> MGYYDDDAHGHVEADAAPRATTGTGTGSASQTVTIPCHHIRLGDILILQGRPCQVIRISTSAATGQHRYLGVDLFTKQLHEESSFVSNPAPSVVVQTMLGPVFKQYRVLDMQDGSIVAMTETGDVKQNLPVIDQSSLWNRLQKAFESGRGSVRVLVVSDHGREMAVDMKVVHGSRLA

Here, we present InCellCryst, an advanced pipeline for producing homogeneous microcrystals directly within living insect cells. We have demonstrated the pipeline on five different proteins (IMPDH, HEX-1, Cathepsin B, Luciferase and EGFP-µNS), representing a selection of soluble proteins of different source organisms that crystallize in insect cells in their native compartment or, in case of peroxisomes, readily in the cytoplasm or nucleus of the cells. Importantly, as shown for IMPDH and HEX-1, InCellCryst can produce crystals from native protein sequences, without purification tags or even remnants of proteolytically removed tags, within a quasi-native cellular environment. The rich source of biomolecules in the cellular environment allows the identification of native ligands by co-crystallization at quasi physiological conditions, representing a unique feature of InCellCryst.

The N- and C-terminal addition of single amino acids (cyto) leads to spindle-like crystals in the cytosol. The disruption of the native PTS1 signal by cloning into the pFB1 cyto and cyto v2 vectors transformed the hexagonal crystal blocks into a spindle-like shape. Whereas HEX-1 cyto and cyto v2 both formed spindle-like as well as bipyramidal crystals, HEX-1 ori crystals exhibit a hexagonal block shape. For HEX-1 ori and HEX-1 cyto crystals diffracted at 100 K one distinct unit cell population was found, whereas two unit cell populations were identified for HEX-1 cyto v2. For data collection from intact crystal-containing cells at 100 K, we carefully transferred the cells onto a MicroMesh mounted on a light microscope stage. Serial diffraction datasets of the crystals contained in viable cells was performed using a helical grid scan approach, available at the EMBL P14 beamline located at the PETRA III storage ring (DESY, Hamburg, Germany). CrystFEL is optimized for still images in high multiplicity collected at RT at XFEL sources and thus, can be directly applied to serial synchrotron data. All HEX-1 structures show an increased flexibility between Phe145 and Ser151, the C-terminal loop region after the α-helix.[(2R,3S,4R,5R)-5-(6-AMINO-9H-PURIN-9-YL)-4-HYDROXY-3-(PHOSPHONOOXY)TETRAHYDROFURAN-2-YL]METHYL (3R)-3-HYDROXY-4-{[3-({2-[(2-HYDROXYETHYL)DITHIO]ETHYL}AMINO)-3-OXOPROPYL]AMINO}-2,2-DIMETHYL-4-OXOBUTYL DIHYDROGEN DIPHOSPHATE | C23 H40 N7 O17 P3 S2 | 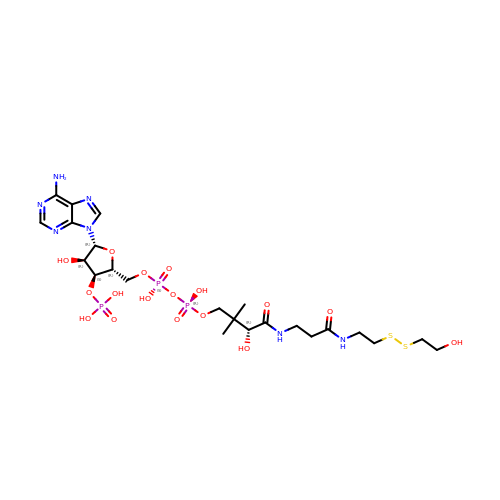MQCDRNSLNTXXSJ-ZSJPKINUSA-N>ATCANGKTVGDASCCAWFDVLDDIQANMFHGGQCGAEAHESIRLVFHDSIAISPAMEAKGKFGGGGADGSIMIFDTIETAFHPNIGLDEVVAMQKPFVQKHGVTPGDFIAFAGAVALSNCPGAPQMNFFTGRKPATQPAPDGLVPEPFHTVDQIIARVNDAGEFDELELVWMLSAHSVAAVNDVDPTVQGLPFDSTPGIFDSQFFVETQFRGTLFPGSGGNQGEVESGMAGEIRIQTDHTLARDSRTACEWQSFVG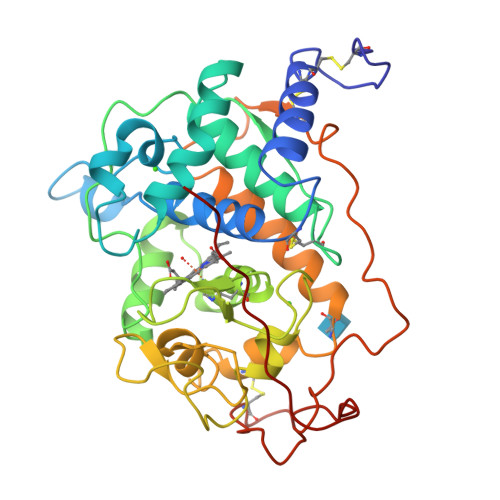NQSKLVDDFQFIFLALTQLGQDPNAMTDCSDVIPLSKPIPGNGPFSFFPPGKSHSDIEQACAETPFPSLVTLPGPATSVARIPPHKA[2x]> MLPVLWLESADTDLDDITSYIARFDIDAAERLWQRLRGCVLPLS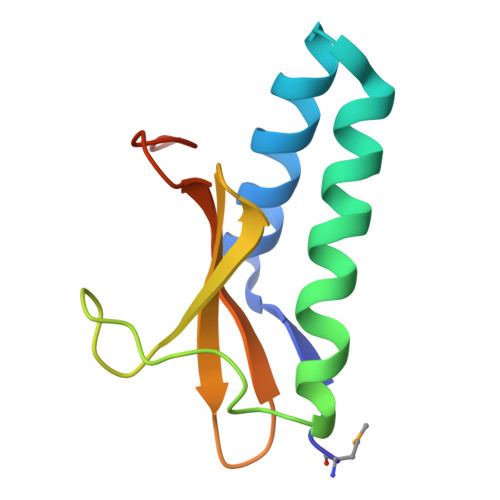EHPYLYPPSDRVPGLREIVAHPNYIILYRVTTSSVEVVNVIHARRQFPLEHHHHHH>[10x]AERLCHPCPWEWTFFQGNCYFMSNSQRNWHDSITACKEVGAQLVVIKSAEEQNFLQLQSSRSNRFTWMGLSDLNQEGTWQWVDGSPLLPSFKQYWNRGEPNNVGEEDCAEFSGNG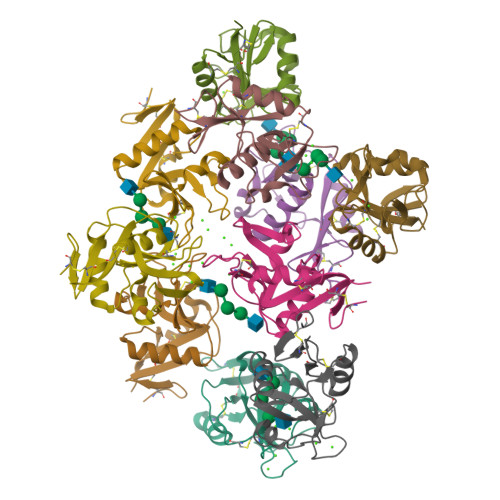WNDDKCNLAKFWICKKSAASCSRDEEQFLSPAPATPNPPPA> PMSRAYDLVVLGAGSGGLEAGWNAAVTHKKKVAVVDVQATHGPPLFAALGGTCVNVGCVPKKLMVTGAQYMDLIRESGGFGWEMDRESLCPNWKTLIAAKNKVVNSINESYKSMFADTEGLSFHMGFGALQDAHTVVVRKSEDPHSDVLETLDTEYILIATGSWPTRLGVPGDEFCITSNEAFYLEDAPKRMLCVGGGYIAVEFAGIFNGYKPCGGYVDLCYRGDLILRGFDTEVRKSLTKQLGANGIRVRTNLNPTKITKNEDGSNHVHFNDGTEEDYDQVMLAIGRVPRSQALQLDKAGVRTGKNGAVQVDAYSK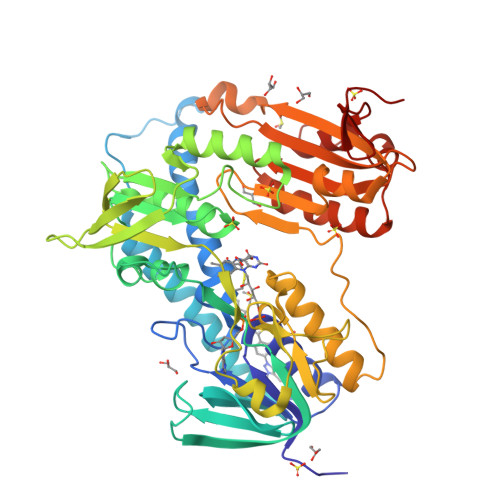TSVDNIYAIGDVTNRVMLTPVAINEGAAFVETVFGGKPRATDHTKVACAVFSIPPIGTCGMTEEEAAKNYETVAVYASSFTPLMHNISGSKHKEFMIRIITNESNGEVLGVHMLGDSAPEIIQSVGICMKMGAKISDFHSTIGVHPTSAEELCSMRTPAYFYESGKRVEKLS> GMLPPVGVQAVALTHDAVRVSWADNSVPKNQKTSEVRLYTVRWRTSFSASAKYKSEDTTSLSYTATGLKPNTMYEFSVMVTKNRRSSTWSMTAHATTYEAAPTSAPKDLTVITREGKPRAVIVSWQPPLEANGKITAYILFYTLDKNIPIDDWIMETISGDRLT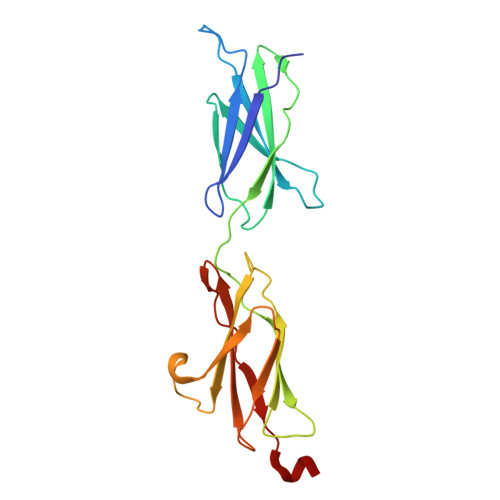HQIMDLNLDTMYYFRIQARNSKGVGPLSDPILFRTLKLEVLFQ>[8x]MSDEAERQRGNNLYKNSPLLPVSISQVSTSQLRETEIMSTNINLFSSYQLGELELPNRIVMAPLTRQRAGEGNVPHQLNAIYYGQRASAGLIIAEATQVTPQGQGYPHTPGIHSPEQVAGWKLVTDTVHQQGGRIFLQLWHVGRISHPDLQPDGGLPVAPSAIAPKGEVLTYEGKKPYVTPRALDTSEIP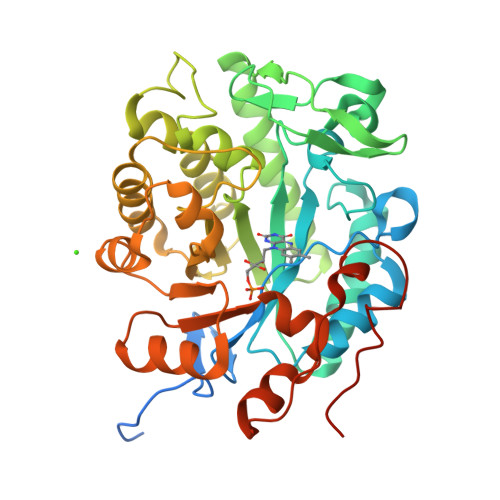AIVEQYRQGAANALAAGFDGVEIHAANGYLIDQFLRDGTNQRTDEYGGAIENRARLLLEVTEAITSVWDSQRVGVRLSPSGTFNDIRDSHPLETFGYVAQALNRFNLSYLHIFEAIDADIRHGGTVVPTSHLRDRFTGTLIVNGGYTREKGDTVIANKAADLVAFGTLFISNPDLPERLEVNAPLNQADPTTFYGGGEKGYTDYPFLAVANKLEHHHHHH2-[(2-carboxy-5-nitrophenyl)amino]-3-methylbenzoic acid | C15 H12 N2 O6 | 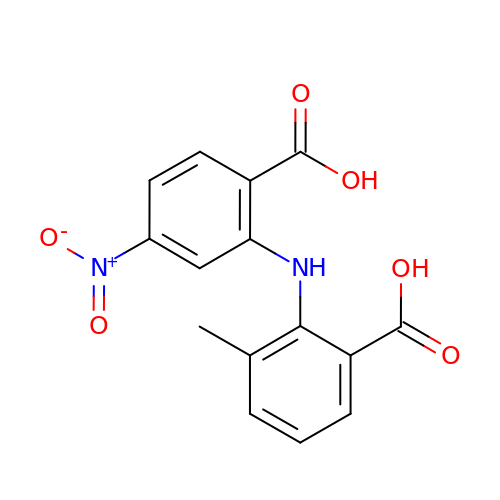LKOWRACJCMMHTL-UHFFFAOYSA-N> GSMIGIIGAMEEEVTILKNKLTQLSEISVAHVKFYTGILKDREVVITQSGIGKVNAAISTTLLINKFKPDVI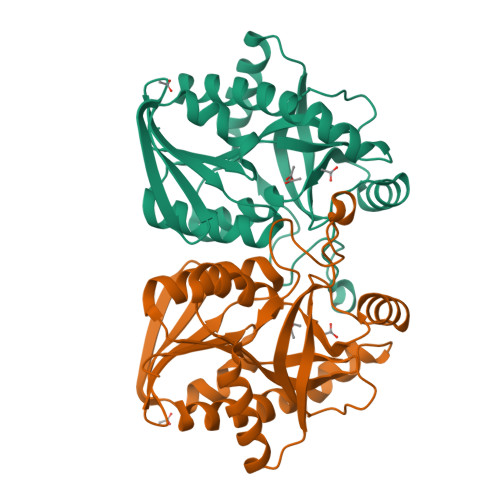INTGSAGALDESLNVGDVLISDDVKYHDADATAFGYEYGQIPQMPVAFQSSKPLIEKVSQVVQQQQLTAKVGLIVSGDSFIGSVEQRQKIKKAFPNAMAVEMEATAIAQTCYQFNVPFVVVRAVSDLANGEAEMSFEAFLEKAAVSSSQTVEALVSQL> SKSDPFSRLKTRTKVYYQE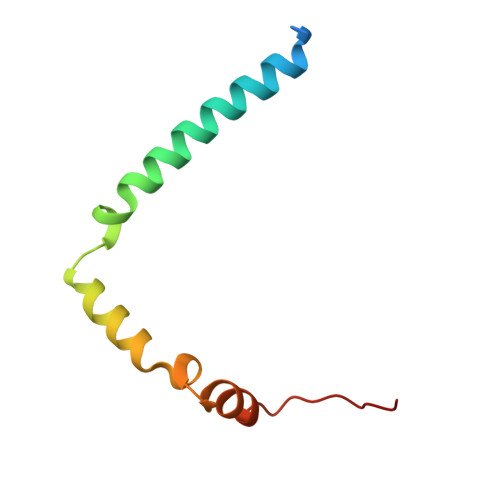IQKEENAKAKEMAQQEKLQEDRETKERREKELLLAQFRRLGGLERMIGELDIKFDFKF>[4x]SMALASKTAIVTGAARGIGFGIAQVLAREGARVIIADRDAHGEAAAASLRESGAQALFISCNIAEKTQVEALFSQAEEAFGPVDILVNNAGINRDAML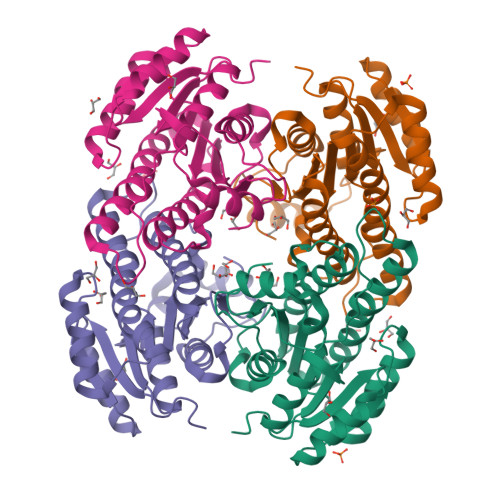HKLTEADWDTVIDVNLKGTFLCMQQAAIRMRERGAGRIINIASASWLGNVGQTNYSASKAGVVGMTKTACRELAKKGVTVNAICPGFIDTDMTRGVPENVWQIMISKIPAGYAGEAKDVGECVAFLASDGARYINGEVINVGGGMVL>[2x]GSADFTETFESSTHGEAPAEWTTIDADGDGQGWLCLSSGQLDWLTAHGGSNVVSSFSWNGMALNPDNYLISKDVTGATKVKYYYAVNDGFPGDHYAVMISKTGTNAGDFTV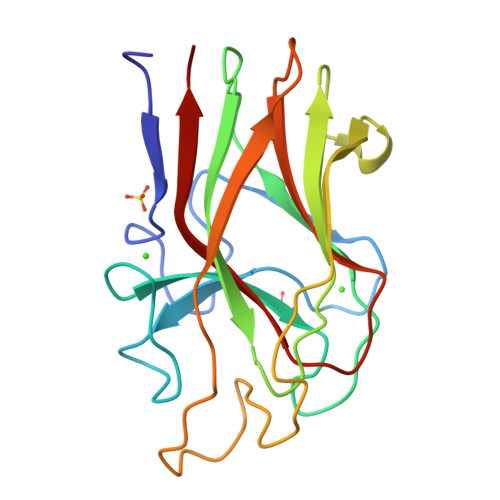VFEETPNGINKGGARFGLSTEANGAKPQSVWIERTVDLPAGTKYVAFRHYNCSDLNYILLDDIQFTMGG>GRVYYINSHGTLSRHENTLRFENAEVKKDIPVEDVEEIFVFAELSLNTKLLNFLA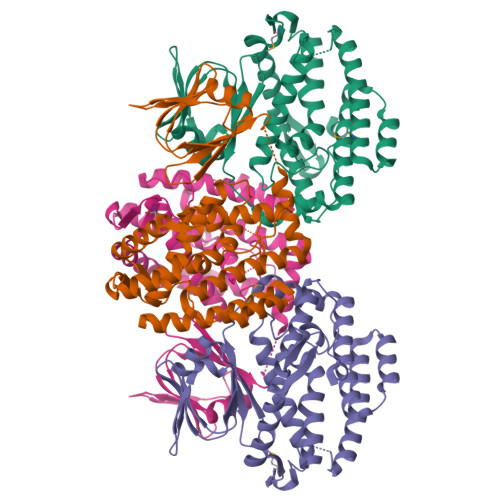SKGIPLHFFNYYGYYTGTFYPRESSVSGHLLIKQVEHYLDAQKRLYLAKSFVIGSILNLEYVYKISADTYLNKVKETNSIPELMSVEAEFRKLCYKKLEEVTGWELEKRTKRPPQNPLNALISFGNSLTYAKVLGEIYKTQLNPTVSYLHEPSTKRFSLSLDVAEVFKPIFVDNLIIRLIQENKIDKTHFSTELNMTFLNEIGRKVFLKAFNELLETTIFYPKLNRKVSHRTLIKLELYKLIKHLLEEEVYLPLNYGGLK[2x]> GASQFFKDNCNRTTASLVEGVELTKYISDINNNTDGMYVVSSTGGVWRISRAKDYPDNVMTAEMRKIAMAAVLSGMRVNMCASPASSPNVIWA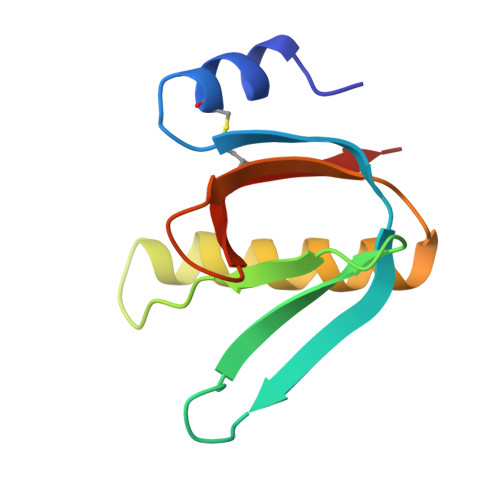IELEAE>[2x]MSIIHVTDDSFDQDVLKADKPVLVDFWAEWCGPCKMIAPILDEIAEE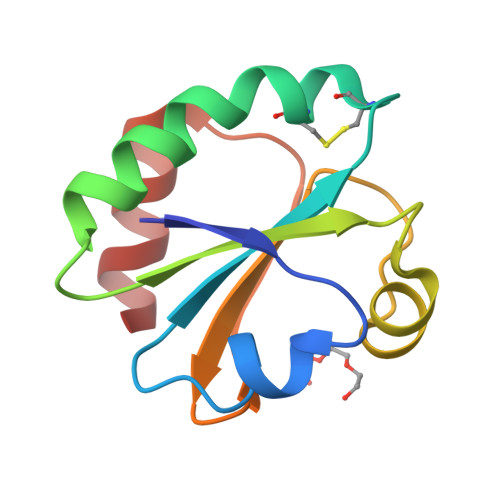YEGKLKVAKVNIDENPETAAKYGIRGIPTLMLFKNGEVAATKVGALSKSQLKEFLDANL> MARKRTSKNDPLRMYLNYVRKLQTMGDAYDESAKYRIANFENGFKSLHMVENEFK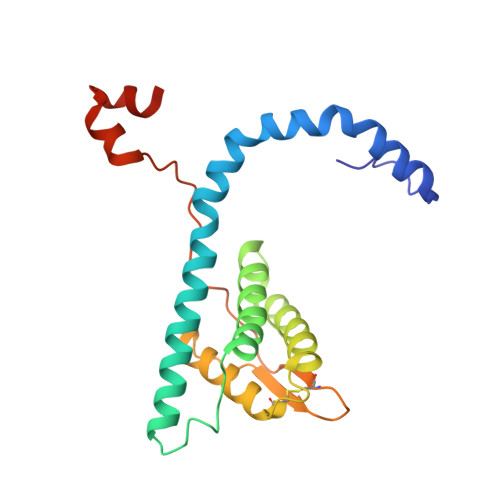QYLANVIDEAIKSGASPQDLPYVNEIKLALMKIFTSWLKYSNEKLGANEIAINVAGTATMTLTENLYGTRVSCEEAVSLINSIFAVWVGVEPFEAEEREGACLVTPRSPLPPVPISSPTGFSAPIQEVLQAKSPEEIIGVKGGA> VKPLQVEPPEPVVAVALGASRQLTCRLACADRGASVQWRGLDTSLGAVQSDTGRSVLTVRNASLSAAGTRVCV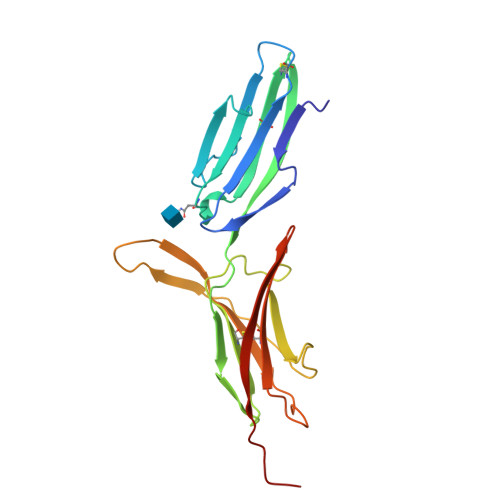GSCGGRTFQHTVQLLVYAFPNQLTVSPAALVPGDPEVACTAHKVTPVDPNALSFSLLVGGQELEGAQALGPEVQEEEEEPQGDEDVLFRVTERWRLPPLGTPVPPALYCQATMRLPGLELSHRQAIPVLHSPTSPE>[2x]TRTYDREGFKKRAACLCFRSEQEDEVLLVSSSRYPDQWIVPGGGMEPEEEPGGAAVREVYEEAGVKGKLGRLLGIFENQDRKHRTYVYVLTVTE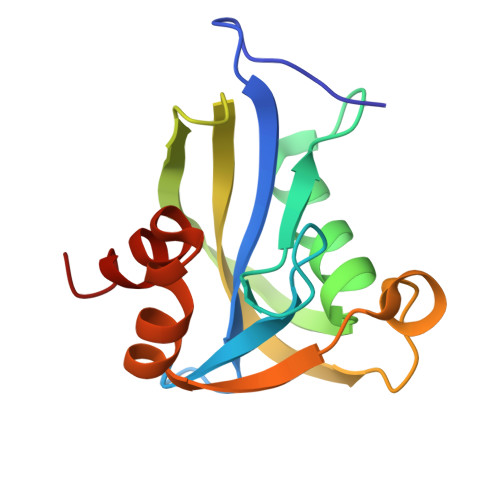ILEDWEDSVNIGRKREWFKVEDAIKVLQCHKPVHAEYLEKLKLG Human tyrosyl-DNA phosphodiesterase 1 (TDP1) is a 608 amino acid DNA repair enzyme that processes 3′-DNA end-blocking lesions by hydrolyzing the 3′-phosphate esters. TDP1 is of importance because it can reverse stalled type I topoisomerase (TOP1)-DNA cleavage complexes (TOP1cc′s) by cleaving the phosphodiester bond between the TOP1 Y723 residue and the 3′-phosphate of its DNA substrate (Pommier, 2006; 2009). When acting on TOP1cc′s, the target phosphate ester bond nestles in a well-formed pocket that contains the signature “His-Lys-Asn” (HKN) catalytic residues. As we report herein, we have designed phosphonic acid-containing variants of our previously reported carboxylic acid-containing imidazopyrazine and imidazopyridine inhibitors and we have obtained crystal structures of the catalytic domain of TDP1 (148–608) complexed with a subset of these inhibitors.

In our current work, we obtained X-ray diffraction data from crystals soaked with compounds 3b and 4c at 1.56 Å and 1.58 Å resolution, respectively. Unambiguous electron density for compound 4c was observed in chain B of TDP1 while the active site pocket of chain A had no compound bound. Compound 4c was observed to bind to the active site of TDP1 with the benzylphosphonic acid headgroup nestled at the base of pocket lined with the catalytic residues. Direct hydrogen bonding interactions are observed between the phosphonic acid 03 oxygen and the of the side chain nitrogen atoms of N283 (3.0 Å) and H493 (2.7 Å). Additional binding interactions occur via a network of water-mediated hydrogen bonds between the 03 oxygen of the phosphonic headgroup and water 828 (2.9 Å) with the side chains of K265 (2.6 Å) and H263 (3.2 Å). The 04 oxygen atom of the phosphonic acid headgroup, however, does not hydrogen bond to any of the active site residues. The Y204 side chain stacks against the aryl moiety of compound 4c via a hydrophobic interaction. Additional hydrophobic interactions occur between the side chain of P461 with the phenyl ring of 4c and W590 with the imidazopyridine. In compound 3b, the phosphonic acid headgroup is positioned approximately at the center of the HKN motif while the phosphonic acid of 4c is shifted approximately 2.6 Å (with respect to the phosphate atom) towards the H493 and K495 residues in comparison with 3b. The phosphonic acid of 4c superimposes closely with the hydroxyl group of the Y723 side chain from the bound TOP1-derived peptide that is covalently attached to the vanadate (which mimics the transition state).

>SGEGQDIWDMLDKGNPFQFYLTRVSGVKPKYNSGALHIKDILSPLFGTLVSSAQFNYCFDVDWLVKQYPPEFRKKPILLVHGDKREAKAHLHAQAKPYENISLCQAKLDIAFGTHHTKMMLLLYEEGLRVVIHTSNLIHADWHQKTQGIWLSPLYPRIADGTHKSGESPTHFKADLISYLMAYNAPSLKEWIDVIHKHDLSETNVYLIGSTPGRFQGSQKDNWGHFRLKKLLKDHASSMPNAESWPVVGQFSSVGSLGADESKWLCSEFKESMLTLGKESKTPGKSSVPLYLIYPSVENVRTSLEGYPAGGSLPYSIQTAEKQNWLHSYFHKWSAETSGRSNAMPHIKTYMRPSPDFSKIAWFLVTSANLSKAAWGALEKNGTQLMIRSYELGVLFLPSAFGLDSFKVKQKFFAGSQEPMATFPVPYDLPPELYGSKDRPWIWNIPYVKAPDTHGNMWVPS[2x]> IEMKPHPWFFGKIPRAKAEEMLSKQRHDGAFLIRESESAPGDFSLSVKFGN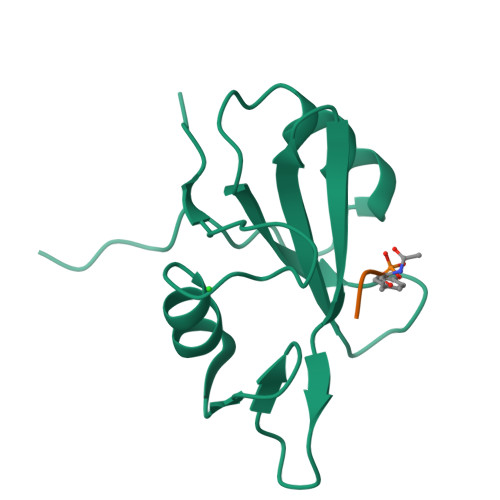DVQHFKVLRDGAGKYFLWVVKFNSLNELVDYHRSTSVSRNQQIFLRDIEQVPQQPTYVQANNNNNN>MATLQDIGVSAGINILSAFVFFIIFAVLRLQPFNDRVYFSKWYLKGLRSSPARGGAFAQRFVNLDFRSYMKFLNWMPEALKMPEPELIDHAGLDSVVYLRIYWLGLKIFTPIAVLAWAVLVPVNWTNNTLEMAKQLRNVTSSDIDKLSVSNIPEYSMRFWTHIVMAYAFTIWTCYVLMKEYETIANMRLQFVASEARRPDQFTVLVRNVPPDADESVSELVEHFFLVNHPDHYLTHQVVCNANKLADLVKKKKKLQNWLDYYQLKYARNNSQRIMVKLGFLGLWGQKVDAIEHYIAEIDKISKEISKEREEVVNDPKAIMPAAFVSFKTRWAAAVCAQTQQTRNPTQWLTEWAPEPRDVFWSNLAIPYVSLTVRRLIMHVAFFFLTFFFIVPIAFVQSLATIEGIVKAAPFLKFIVDDKFMKSVIQGFLPGIALKLFLAFLPSILMIMSKFEGFTSISSLERRAAFRYYIFNLVNVFLASVIAGAAFEQLNSFLNQSANQIPKTIGVAIPMKATFFITYIMVDGWAGVAGEILMLKPLIMFHLKNAFLVKTDKDREEAMDPGSIGFNTGEPRIQLYFLLGLVYAPVTPMLLPFILVFFALAYIVYRHQIINVYNQEYESAAAFWPDVHGRVIAALVISQLLLMGLLGTKHAALAAPFLIALPVLTIGFHHFCKGRYEPAFIRYPLQEAMMKDTLETAREPNLNLKGYLQNAYVHPVFKGDEDDYDIDDKLGKFEDEAIIVPTKRQSRRNTPAPSIISGDDSPSLPFSGKLV[2x]

Via genetic screens and functional analysis, the osmosensitive Ca2+ permeable cation channel proteins were identified in Arabidopsis by two independent groups, which was named CSC1 (alias OSCA1.2 according to the OSCA family nomenclature that is used here) and OSCA1, respectively. OSCA1.2 and OSCA1 share ~85% sequence identity, and they both can be activated by hyperosmolality treatment. In addition to Ca2+, they are also permeable to monovalent cations such as Na+ and K+, suggesting low cation selectivity. Members of the OSCA family belong to the calcium-permeable stress-gated cation channel family (entry number of 1.A.17.5 in Transporter Classification Database), a subfamily of the calcium-dependent chloride channel (Ca-ClC) family.

Here, we present the structure of OSCA1.2 from Arabidopsis thaliana (AtOSCA1.2) determined by single-particle cryo-electron microscopy (cryo-EM) with a nominal resolution of 3.68 Å for the overall structure. AtOSCA1.2 forms a homodimer, similar to nhTMEM16 and mTMEM16A. Each monomer contains 11 transmembrane helices, in contrast to nhTMEM16 and mTMEM16A, which have only 10 TMS. In contrast to nhTMEM16 and mTMEM16A, of which the dimer formation is mediated by direct interaction between the transmembrane helices TM3 and TM10, the dimer interface of AtOSCA1.2 is exclusively formed by its cytosolic domain. Despite the separate biological functions and low sequence similarity between the AtOSCA1.2 and TMEM16 proteins (~11% sequence identity between AtOSCA1.2 and mTMEM16A), structural alignments reveal that the last 10 TMS of AtOSCA1.2 share a similar fold with nhTMEM16 and mTMEM16A. The ion conduction pore of AtOSCA1.2 is in a closed state in the solved structure, as revealed by pore radius analysis. The conduction pore is constricted by a set of hydrophobic residues, which include I393 on TM4, L434 and L438 on TM5, V476 on TM6, F515, F516 and Y519 on TM7 and L575 and L579 on TM8. We have also identified two long helices in the cytosolic domain of AtOSCA1.2 that lie parallel to the membrane plane (named ICα2 and ICα3). In AtOSCA1.2, the hydrophobic linker between the two long cytosolic helices is identified as an unique structural component and may serve as a sensor of osmotic stress. In the structure, this linker protrudes into the lipid bilayer as an anchor, and its partial deletion impairs the opening of the channel under hyperosmotic stress.>[2x]MSLKILDCTLRDGGYYTNWDFNSKIVDAYILA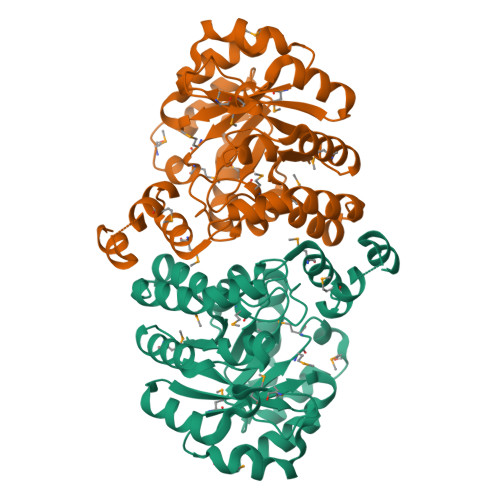MNELPIDYLEVGYRNKPSKEYMGKFGYTPVSVLKHLRNISTKKIAIMLNEKNTTPEDLNHLLLPIIGLVDMIRIAIDPQNIDRAIVLAKAIKTMGFEVGFNVMYMSKWAEMNGFLSKLKAIDKIADLFCMVDSFGGITPKEVKNLLKEVRKYTHVPVGFHGHDNLQLGLINSITAIDDGIDFIDATITGMGRGAGNLKMELLLTYLNKHHGLNVDFNVLGNIITTFTPLLEKYQWGTNLPYMLSGANNIPQKEVMDWVTNRVYSFNSIIRALDNRKNKMEEGHHHHHH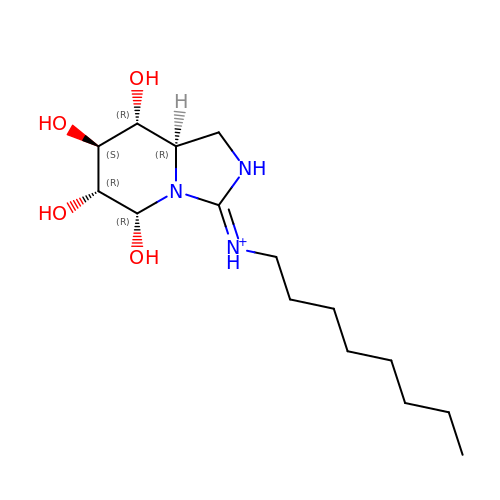N-[(3E,5R,6R,7S,8R,8AR)-5,6,7,8-TETRAHYDROXYHEXAHYDROIMIDAZO[1,5-A]PYRIDIN-3(2H)-YLIDENE]OCTAN-1-AMINIUM | C15 H30 N3 O4 | DGGJYTDCPYQDLL-RKQHYHRCSA-O>[3x]CVIFPVEIDVSQTIIRDCQVDKQTRELVYINKIMNTMLTKPVLMMFNISGPIRSVTRKNNNLRDRIKSKPDEQFDQLERDYSDQMDGFHDSIKYFKDEHYSVSCQNGSVLKSKFAKILKSHDYTDKKSIEAYEKYCLPKLVDERNDYYVAVCVLKPGFENGSNQVLSFEYNPIGNKVIVPFAHEINDTGLYEYDVVAYVDSVQFDGEQFEEFVQSLILPSSFKNSEKVLY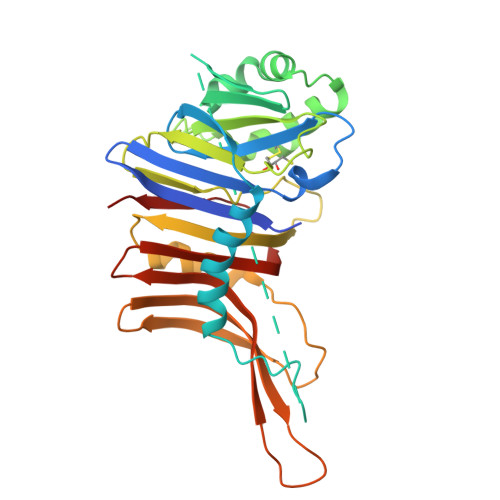YNEASKNKSMIYKALEFTTESSWGKSEKYNWKIFCNGFIYDKKSKVLYVKLHNVTSALNKNVILNTIK> RAPDSVDYRKKGYVTPVKNQGQCGSCWAFSSVGALEGQLKKKTGKLLNLSPQNLVDCVSENDGCGGGYMTNAFQYVQKNRGIDSEDAYPYVGQEESCMYNPTGKAAKCRGYREIPEGNEKALKRAVARVGPVSVAIDASLTSFQFYSKGVYYDESCNSDNLNHAVLAVGYGIQKGNKHWIIKNSWGENWGNKGYILMARNKNNACGIANLASFPKM;> LYPEEILDTHWELWKKTHRKQYNNKVDEISRRLIWEKNLKYISIHNLEASLGVHTYELAMNHLGDMTSEEVVQK

Cathepsin K (CatK) is one of the most investigated cysteine cathepsins, both by academia and pharmaceutical companies. It is expressed in high levels in osteoclasts, where it serves as the principal protease involved in bone remodelling. Cathepsin K (CatK) is a target for the treatment of osteoporosis, arthritis, and bone metastasis. Peptidomimetics with a cyanohydrazide warhead represent a new class of highly potent CatK inhibitors; however, their binding mechanism is unknown.

The obtained iCatK comprised two non-covalently bound domains (chains), namely the residual propeptide domain (Glu5p to Ser83p) and the main domain (Ser87p to Met215), including the C-terminal part of the propeptide and mCatK. The model of the iCatK-Gü2602 complex contained residues Asp8p to Lys74p and Arg99p to Met215. The propeptide segment that blocks the active site in pCatK (downstream of the α3p helix) is proteolytically removed or flexible in iCatK, and therefore the active site cleft of iCatK becomes accessible for inhibitors. However, the residual propeptide domain partially occludes the primed region of the active site, in particular the S1’ subsite of iCatK is occupied. In general, Gü2602 binds to the S1 and S2 subsites of iCatK in a manner that is similar to what has been shown for the Gü2602-mCatK complex, with a r.m.s.d. of 1.23 Å; this value is substantially increased compared to Gü1303 in its complexes, with a r.m.s.d. of 0.19 Å. The major conformational change, however, is in the benzyl group of the P1 N-benzyl-N-methylacetamide substructure. It is rotated towards the residual propeptide domain of iCatK and forms new contacts with its Val72p and Gln73p residues (Figure 5(A,B), Table S2). The terminal Boc group accommodates the S2 pocket of iCatK analogously as in mCatK. The network of hydrogen bonds is identical, and the pattern of nonpolar interactions (Tyr67, Asn161, and Ala163 in iCatK) is similar for both Gü2602 complexes. iCatK was demonstrated to bind Gü2602 and Gü1303 in an analogous manner to that observed in the mCatK complexes. This indicated that the iCatK active site is competent to bind inhibitory ligands in the available subsites and can be regulated by them.N-ISOPROPYL-N'-HYDROXYGUANIDINE 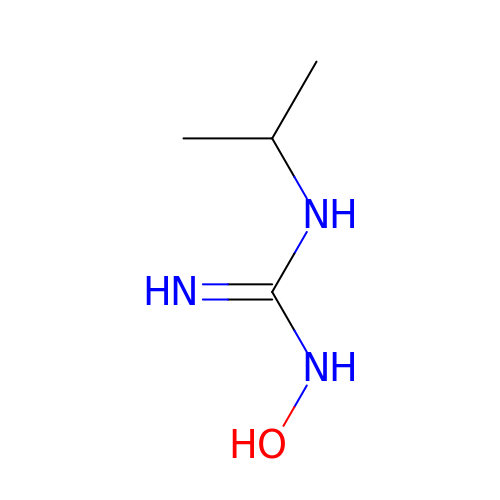| C4 H11 N3 O | OITVEDMMUMUWTL-UHFFFAOYSA-N DIHYDROFLAVINE-ADENINE DINUCLEOTIDE | C27 H35 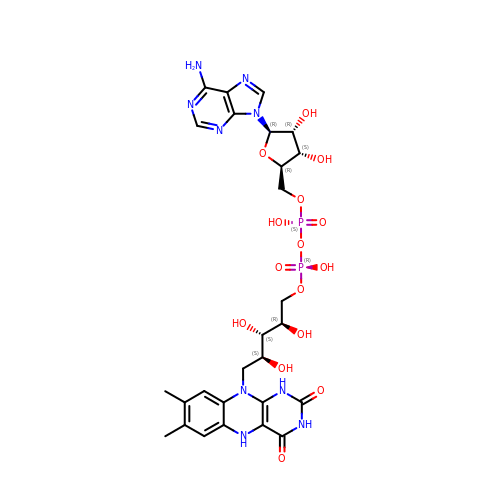N9 O15 P2 | YPZRHBJKEMOYQH-UYBVJOGSSA-N>SLFKDDIQLNEHQVAWYSKDWTAVQSAADSFKEKAENEFFEIIGAINNKTKCSIAQKDYSKFMVENALSQFPECMPAVYAMNLIGSGLSDEAHFNYLMAAVPRGKRYGKWAKLVEDSTEVLIIKLLAKRYQVNTNDAINYKSILTKNGKLPLVLKELKGLVTDDFLKEVTKNVKEQKQLKKLALEWGLEHHHHHHHHHH[2x];>GPGGSMITVNEKEHILEQKYRPSTIDECILPAFDKETFKSITSKGKIPHIILHSPSPGTGKTTVAKALCHDVNADMMFVNGSDCKIDFVRGPLTNFASAASFDGRQKVIVIDEFDRSGLAESQRHLRSFMEAYSSNCSIIITANNIDGIIKPLQSRCRVITFGQPTDEDKIEMMKQMIRRLTEICKHEGIAIADMKVVAALVKKNFPDFRKTIGELDSYSSKGVLDAGILSLVTNDRGAIDDVLESLKNKDVKQLRALAPKYAADYSWFVGKLAEEIYSRVTPQSIIRMYEIVGENNQYHGIAANTELHLAYLFIQLACEMQWK[8x];>MKLSKDTTALLKNFATINSGIMLKSGQFIMTRAVNGTTYAEANISDVIDFDVAIYDLNGFLGILSLVNDDAEISQSEDGNIKIADARSTIFWPAADPSTVVAPNKPIPFPVASAVTEIKAEDLQQLLRVSRGLQIDTIAITVKEGKIVINGFNKVEDSALTRVKYSLTLGDYDGENTFNFIINMANMKMQPGNYKLLLWAKGKQGAAKFEGEHANYVVALEADSTHDF[6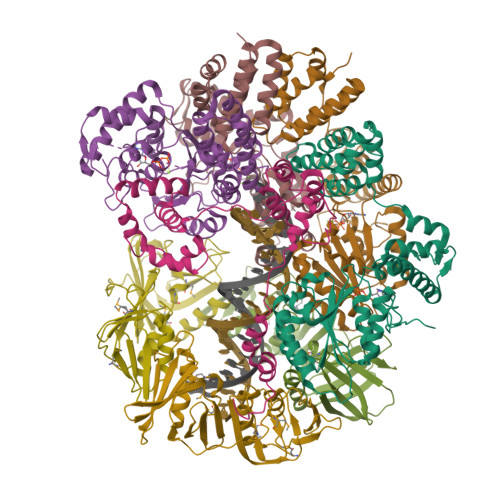x]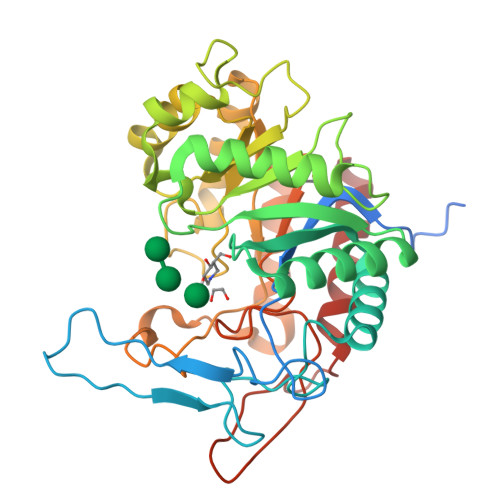> MMIFFLSLSLESCSKEDDNNPSNSENNGGNNNLGTELDYDTFCFYYDWYGSEAIDGQYRHWAHAIAPDPNGGSGQNPGTIPGTQESIASNFYPQLGRYSSSDPNILTKHMDMFVMARTGVLALTWWNEQDETEAKRIGLILDAADKKKIKVCFHLEPYPSRNVQNLRENIVKLITRYGNHPAFYRKDGKPLFFIYDSYLIEPSEWEKLLSPGGSITIRNTAYDALMIGLWTSSPTVQRPFILNAHFDGFYTYFAATGFTYGSTPTNWVSMQKWAKENGKIFIPSVGPGYIDTRIRPWNGSVIRTRTDGQYYDAMYRKAIEAGVSAISITSFNEWHEGSQIEPAVPYTSSEFTYLDYENREPDYYLTRTAYWVGKFRESKQ>[2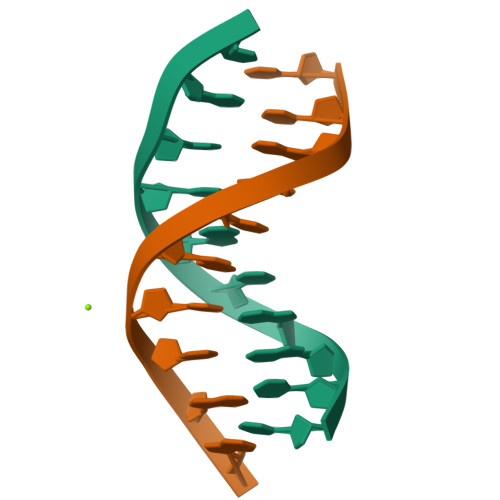x]CCAACITTGG> MHHHHHHSGGSRSEAHSNSIGILAMHNNIIRDFTKIASNNIDLAIEDITTVDHSLNSIYSLLKSHHMWGHINSTVKQHLMIIVKLINNNALGLASSEIIFLFNETNLFQAHSLKNILLADFSTWNDYYLSNLKILALQIILKRKLVDEYLPHILELFSHDKRYLLKDPNLKAHALTKIVLSFFSVTTSCKVLFGLKFLQYIKQFKLPFKKFISNITVECFSKNLLHKNYLEMGPNKIYLNSFYLSYSMLYDGLDKIMLLDILSYEETTEVQRAIKSKKEFNEYCNMSENRLLWSCISVDDLNVILENATNFLQNKGKHISATLKCLVCLWSTIRLEGLPKNKDILRQFDCTVIYINSNIKSINDESAAALLSELLGVLSEICIDYKEPKRLSNIISVLFNASVLFKSHSFLLKTANLEISNVLISNDSKTSHRTILKFEKFISSAQSAQKKIEIFSCLFNVYCMLRNDTLSFVFDFCQNAFIHCFTRLKITKFIEFSNSSEIMLSVLYGNSSIENIPSENWSQLSRMIFCSLRGIFDLDPLELNNTFDKLHLLNKYELLIRIVYLLNLDMSKHLTTNLSKITKLYINKWLQKSDEKAERISSFEMDFVKMLLCYLNFNNFDKLSIELSLCIKSKEKYYSSIVPYADNYLLEAYLS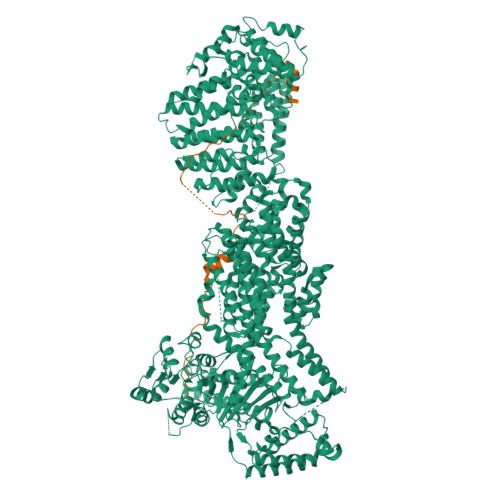LYMIDDALMMKNQLQKTMNLSTAKIEQALLHASSLINVHLWDSDLTAFQIYFGKTLPAMKPELFDINNDHNLPMSLYIKVILLNIKIFNESAKLNIKAGNVISAVIDCRKAQNLALSLLKKKNKLSQGSRLALLKSLSFSFFQLIKIHIRIGSARDCEFYSKELSRIISDLEEPIIVYRCLHFLHRYYMITEQTCLQNITLGKANKAFDYLDAEADITSLTMFLYDNKEFVKLEQSLVLYFGDQLEKTFLPNLWKLHLGKDIDDSICLSEYMPKNVINRVHNMWQKVMSQLEEDPFFKGMFESTLGIPSSLPVIPSTMPNNILKTPSKHSTGLKLCDSPRSSSMTPRGKNIRQKFDRIAAISKLKQMKELLESLKLDTLDNHELSKISSLSSLTLTILSNITSIHNAESSLITNFSLTDLPRHMPLLFDKVLNNIDNKNYREFRVSSLIAPNNISTITESIRVSAAQKDLMESNLNINVITIDFCPITGNLLLSKLEPRRKRRTHLRLPLIRSNSRDLDEVHLSFPEATKKLLSIINESNQTTSVEVTNKIKTREERKSWWTTRYDLDKRMQQLLNNIENSWFNGVQGFFSPEVVDNSLFEKFKDKFYEILHQNLPSRKLYGNPAMFIKVEDWVIELFLKLNPQEIDFLSKMEDLIYFVLDILLFHGEENAYDEIDFSMLHVQLEEQIKKYRATMTTNSIFHTFLVVSSSCHLFPWECLSFLKDLSITRVPSYVCLNKLLSRFHYQLPLQVTIEDNISMILNPNGDLSRTESKFKGMFQKIIDAKPSSQLVMNEKPEEETLLKMLQNSNLFVYIGHGGGEQYVRSKEIKKCTKIAPSFLLGCSSAAMKYYGKLEPTGTIYTYLLGGCPMVLGNLWDVTDKDIDKFSEELFEKMGFRCNTDDLNGNSLSVSYAVSKSRGVCHLRYLNGAAPVIYGLPIKFVS;> MDIEIAPQRQEPLPYVPEGYSPFQQDDIEKLKTFNSPYKLDLEDEDDTPDKVDLLPLEQIDEEGEKDETECITRNQEEGAALPLLSKNFKEVAAVPTMELVYSEEGLDPEELEDLVT N-(2-AMINOETHYL)-N'-{2-[(2-AMINOETHYL)AMINO]ETHYL}ETHANE-1,2-DIAMINE | C8 H23 N5 | 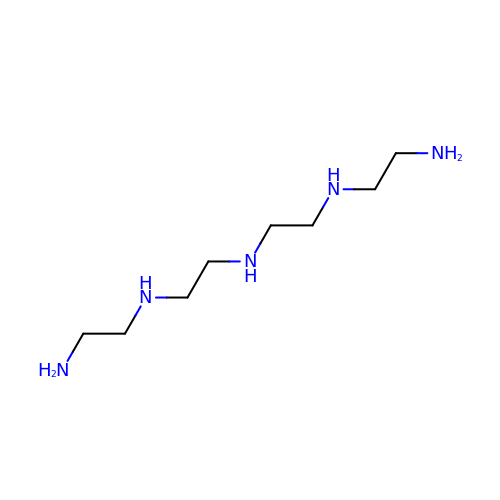FAGUFWYHJQFNRV-UHFFFAOYSA-N> GGACAUAUAAUCGCGUGGAUAUGGCACGCAAGUUUCUACCGGGCACCG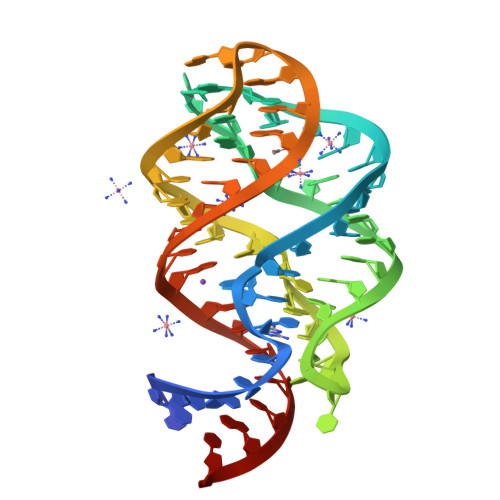UAAAUGUCCGAUUAUGUCC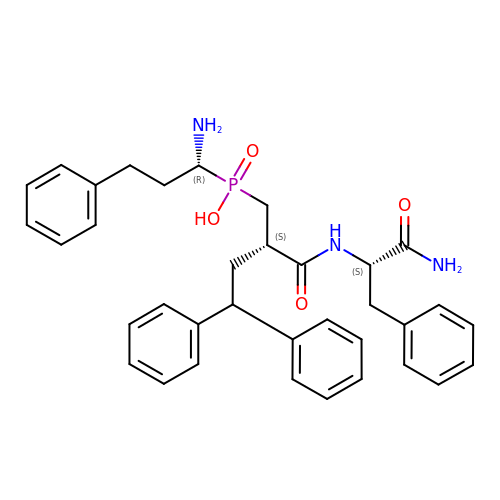[(2~{S})-2-[[(2~{S})-1-azanyl-1-oxidanylidene-3-phenyl-propan-2-yl]carbamoyl]-4,4-diphenyl-butyl]-[(1~{R})-1-azanyl-3-phenyl-propyl]phosphinic acid | C35 H40 N3 O4 P | FDAGDZVCWKCEEX-NGYIUDBNSA-N> MRGSHHHHHHTDPALRAMRLVQLSRHSIAFPSPEGALREPNGLLALGGDLSPARLLMAYQRGIFPWFSPGDPILWWSPDPRAVLWPES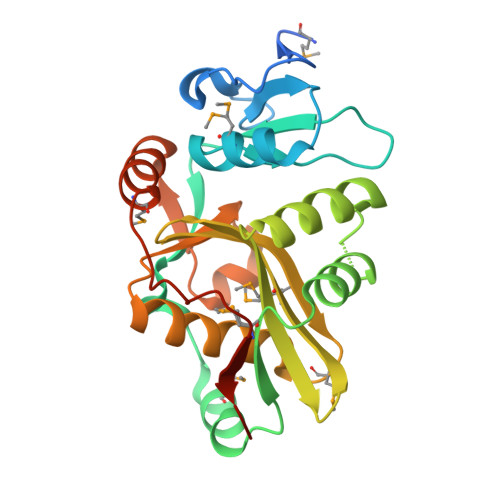LHISRSMKRFHKRSPYRVTMNYAFGQVIEGCASDREEGTWITRGVVEAYHRLHELGHAHSIEVWREDELVGGMYGVAQGTLFCGESMFSRMENASKTALLVFCEEFIGHGGKLIDCQVLNDHTASLGACEIPRRDYLNYLNQMRLGRLPNNFWVPRCLFSPQEGLCGR> SNARDSPY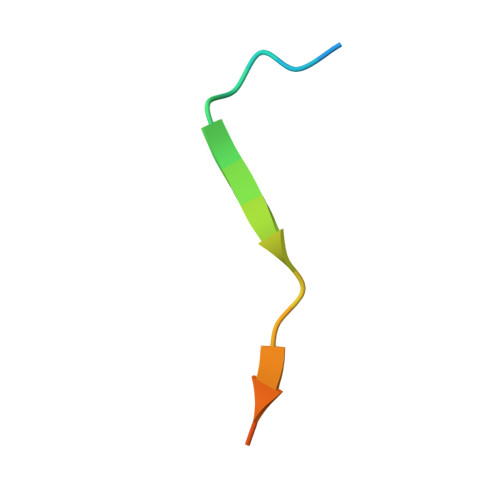GLSQGITKKNKD>[5x]GNQGGFGNSRGGGAGLGNNQGSNMGGG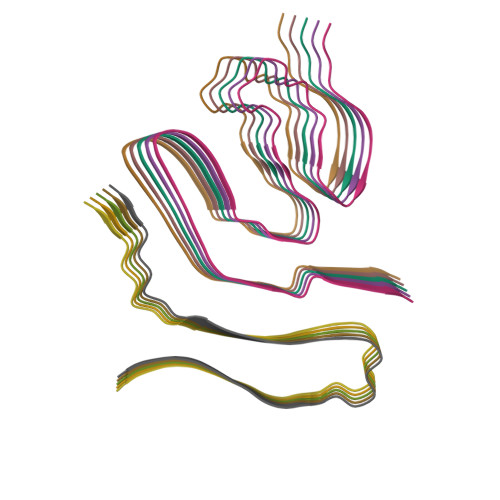MNFGAFSINPAMMAAAQAALQSSWGMMGMLASQQN;>[5x]LDNVATYAGQFNQDYLSGMAANMSGTFGGANMPNLY> MRCSARRANVAALYEFVDGNFLNNKRPAIPGGAWPLESLRRKSLADLQQIWLSLLKERNMLSTIKEHYLRHQEELGAMPAPSRLKMVEESMENVKRVVKERDAEATAEAVRIFKERLAKGIYRYPPGPPPPPGAHDPTSTVKLVLSRRVDEERLRELLGRFNVFEAHKGIVKLTMQLPEDVLTQKRDAEQLWQQYMAERRNVEEYYKWPGSSTGSAESASVYDHTVVELAPGVYSGHRGTSAIESNCVDDSNDGAHGVVQAARLPVPPPKTRPPPPRNPLEHIKY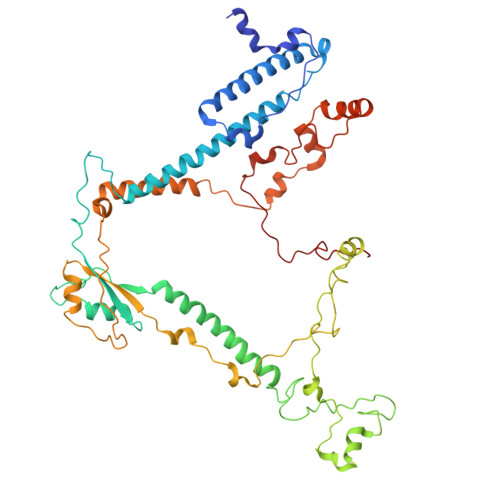QQRSVLSKAVIQLGYFPNITTTAPRFTKADDVPRPVHPDEIEGPWEVRVTYDAKDGLAYVQSLSLTSIDGAAVLSVEEEFPAAAQPYAAVDPVYQEAVRREMAQEETLMKWPNVPKWKYQYDLYTKKHLAQVVQYNYSNVVDYVDREVLLTGRSVWESPIDIDPTCGGMKSVPAHAKKPKRYMTHGLAEVGVTDI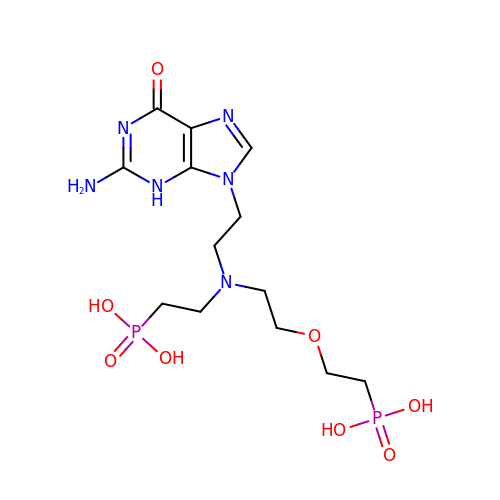(2-{[2-(2-amino-6-oxo-3,6-dihydro-9H-purin-9-yl)ethyl][2-(2-phosphonoethoxy)ethyl]amino}ethyl)phosphonic acid | C13 H24 N6 O8 P2 | ONMAFLJUDYCSLA-UHFFFAOYSA-N Anti-Müllerian hormone (AMH) plays a crucial role in male sex differentiation and female reproductive development. AMH is a member of the transforming growth factor beta (TGF-β) family, which consists of over 30 unique, secreted ligand dimers, divided into three classes based on sequence identity and receptor utilization: TGF-βs, bone morphogenetic proteins (BMPs), and Activins. Remarkably, AMH has evolved within this family to be the only member with its own dedicated type II receptor, AMHR2. To help resolve this question, we solved the crystal structure of the mature C terminus of AMH in complex with the ECD of AMHR2.

Diffraction quality crystals of the AMH/AMHR2 complex were obtained, and the structure was solved to 2.6 Å resolution by molecular replacement. The asymmetric unit contains one AMH monomer and one AMHR2 ECD with the biological complex being generated by crystallographic symmetry, including a disulfide bond that connects the two AMH chains. AMHR2 binds to AMH using the concave surface created by the palm of the receptor, which binds to the convex knuckle surface of AMH. In addition to the central palm–ligand interface, AMHR2 wraps around fingertip 3/4 of AMH through extensions in both fingers 1 and 3 of AMHR2. First, at the center of the interface, there are several hydrophobic residues within the palm of AMHR2, including F62, I64, M76 and L106, which bind to corresponding hydrophobic residues on the knuckle region of AMH (L478, I479, L535, I537, L539, I544, and A546). Second, also centrally located, an unstructured loop within finger 1 of AMHR2 extends toward the interface and creates a short β-parallel interaction with the top of finger 4 of AMH. This positioning facilitates the formation of main-chain hydrogen bonds between residue R33 of AMHR2 and residues I544 and A546 of AMH. Here, a salt bridge is formed between AMHR2 residues D81 and E84 and AMH residue K534. Comparison shows that the receptors are shifted by about 7.5 Å, where the AMHR2 position is shifted toward finger 1/2 of the ligand, while ActRIIA and ActRIIB bind Activins and BMPs toward the top of finger 4. Overall, the structure shows a modified Activin/BMP type II receptor-binding mode, in which AMHR2 is shifted downward and wraps around fingers 3 and 4 of AMH.

> SAGATAADGPCALRELSVDLRAERSVLIPETYQANNCQGVCGWPQSDRNPRYGNHVVLLLKMQARGAALARPPCCVPTAYAGKLLISLSEERISAHHVPNMVATECGCR;> GPHMPPNRRTCVFFEAPGVRGSTKTLGELLDTGTELPRAIRCLYSRCCFGIWNLTQDRAQVEMQGCRDSDEPGCESLHCDPSPRAHPSPGSTLFTCSCGTDFCNANYSHLP SPIRO(2,4,6-TRINITROBENZENE[1,2A]-2O',3O'-METHYLENE-ADENINE-TRIPHOSPHATE | C16 H17 N8 O19 P3 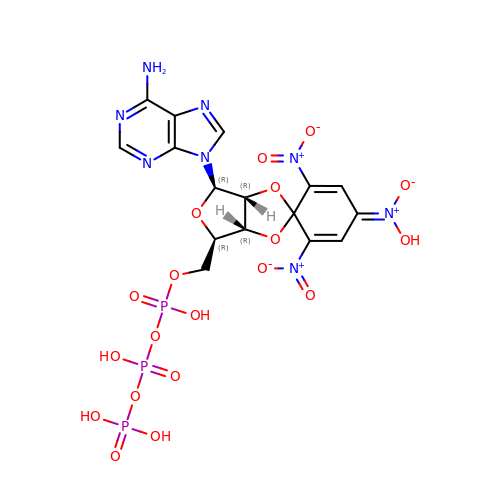| XFMMHXLUHKBKQE-UHEGPQQHSA-N> ALVKEEIQAKEYLENLNKELAKRTNVETEAAWAYGSNITDENEKKKNEISAELAKFMKEVASDTTKFQWRSYQSEDLKRQFKALTKLGYAALPEDDYAELLDTLSAMESNFAKVKVCDYKDSTKCDLALDPEIEEVISKSRDHEELAYYWREFYDKAGTAVRSQFERYVELNTKAAKLNNFTSGAEAWLDEYEDDTFEQQLEDIFADIRPLYQQIHGYVRFRLRKHYGDAVVSETGPIPMHLLGNMWAQQWSEIADIVSPFPEKPLVDVSAEMEKQGYTPLKMFQMGDDFFTSMNLTKLPQDFWDKSIIEKPTDGRDLVCHASAWDFYLTDDVRIKQCTRVTQDQLFTVHHELGHIQY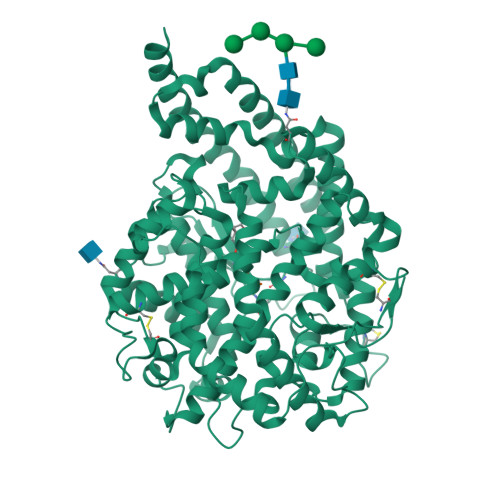FLQYQHQPFVYRTGANPGFHEAVGDVLSLSVSTPKHLEKIGLLKDYVRDDEARINQLFLTALDKIVFLPFAFTMDKYRWSLFRGEVDKANWNCAFWKLRDEYSGIEPPVVRSEKDFDAPAKYHISADVEYLRYLVSFIIQFQFYKSACIKAGQYDPDNVELPLDNCDIYGSAAAGAAFHNMLSMGASKPWPDALEAFNGERIMSGKAIAEYFEPLRVWLEAENIKNNVHIGWTTSNKCVS;> RPPGFTPFR> AVGPVADLTITDAAVSPDGFSRQAVVVNGVTPGPLVAGNIGDRFQLNVIDNLTNHTMLKSTSIHWHGFFQHGTNWADGPAFINQCPISPGHSFLYDFQVPDQAGTFWYHSHLSTQYCDGLRGPFVVYDPNDPHASRYDVDNDDTVITLADWYHTAAKLGPRFPGGADATLING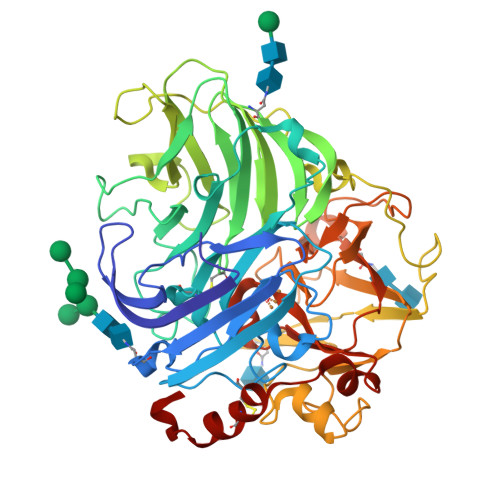KGRAPSDSVAELSVIKVTKGKRYRFRLVSLSCNPNHTFSIDGHNLTIIEVDSVNSQPLEVDSIQIFAAQRYSFVLDANQAVDNYWIRANPNFGNVGFDGGINSAILRYDGAPAVEPTTNQTTSVKPLNEVDLHPLVSTPVPGSPSSGGVDKAINMAFNFNGSNFFINGASFVPPTVPVLLQILSGAQTAQDLLPSGSVYVLPSNASIEISFPATAAAPGAPHPFHLHGHTFAVVRSAGSTVYNYDNPIFRDVVSTGTPAAGDNVTIRFDTNNPGPWFLHCHIDFHLEGGFAVVMAEDTPDVKAVNPVPQAWSDLCPTYDALDPNDQ> SNAMKKVQGIYRAPRQHWVG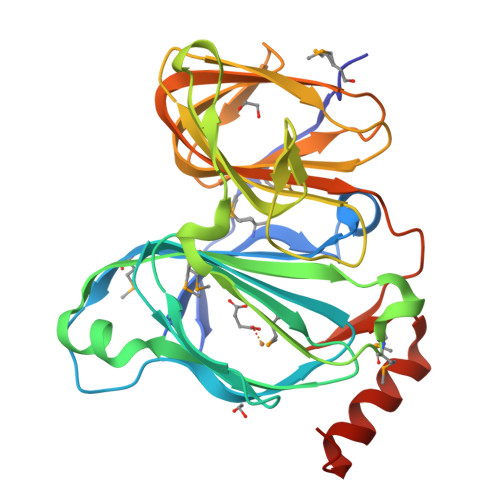DGFPVRSMFSYQSHGKQLSPFLLLDYAGPMDFTPTTQRRGVGQHPHRGFETVTIVYHGEVEHRDSTGNGGIIGPGDVQWMTAGAGILHEEFHSDAFAQKGGPFEMVQLWVNLPAKDKMTAPGYQAIRREAIPQVNLPDDAGNLRVIAGEYAGNIGPAKTFSPLNVWDIRLTQGKSCEFSLPAGWNTALIVLHGTLLVNGDAIAREAEMVLLDPTGTHLSIEANNDTVLLLLSGEPIDEPIVGYGPFVMNTQAQIAEAIADFNGGRFGNMDVA>[4x]NQCPTDWEAEGDHCYRFFNTLTTWENAHHECVSYSCSTLNVRSDLVSVHSAAEQAYVFNYWRGIDSQAGQLWIGLYDKYNEGDFIW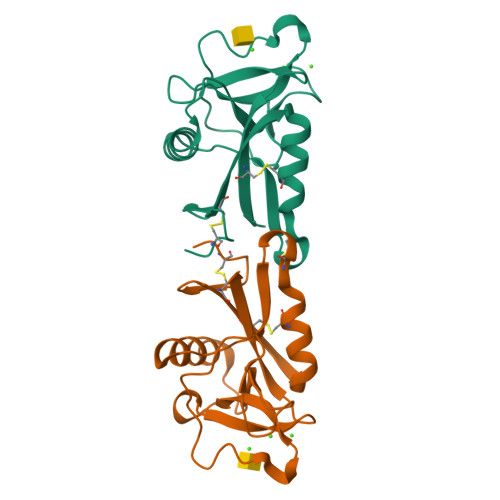TDGSKVGYTKWAGGQPDNWNNAEDYGQFRHTEGGAWNDNSAAAQAKYMCKLTFE>[4x]GAMASYDNVDTLIEKGRYNTKYNYLKRMEKYYPNAMAYFDKVTINPQGNDFYINNPKVELDGEPSMNYLEDVYVGKALLTNDTQQEQKLKSQSFTCKNTD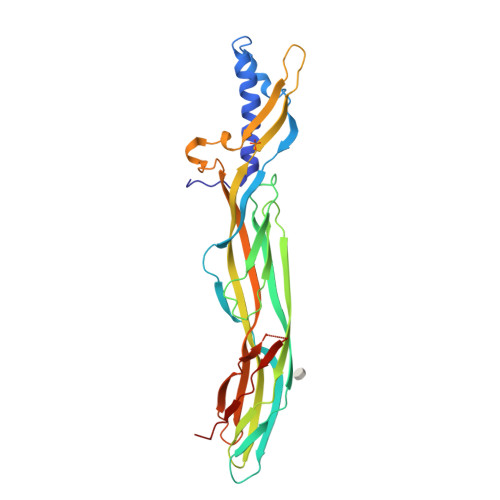TVTATTTHTVGTSIQATAKFTVPFNETGVSLTTSYSFANTNTNTNSKEITANVPSQDILVPANTTVEVIAYLKKVNVKGNVKLVGQVSGSEWGEIPSYLAFPRDGYKFSLSDTVNKSDLNEDGTININGKGNYSAVMGDELIVKVRNLNTNNVQEYVIPVDKIEGRKEKSNDSNIVKYRSLSIKAPGIK> VSNAIKFIILTEIIFPTLLLVFGIYHGVMQVFYRSGIIKAESFLGIDYYQGLTLHGVINVIVYTTIFIVGFSNAIVAYSLKKPLREKVQWIALGMMVIGTLMAAWAMFTGRATVLYTFYPPLIAHWTFYLGAVLLVLGSLVPFFFDWIPSAIQWKRENPDQKLPLAVFGTFVNFILWTIMIVPVAIEILFQLLPLSLGLVDEINPLLARTLFWFFGHPVVYFWLLPAYVALYTILPKIVSEKGKLYSDPAARLAFILFLIFSLPVGLHHQFTDPGITNTWKLIHALFTFGVALPSMITAFTVATSLEYSVKAEHPELKNSKFYWWTFLPFMRLEGNKWMFSYFFAG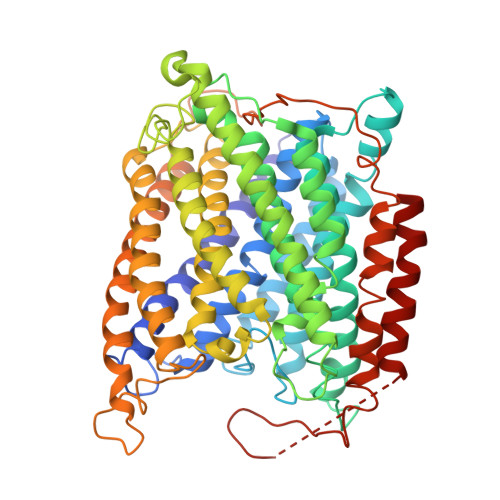LVLFFIGGITGIVNASYNVNLVVHNTAYVPGHFHTTVGGLVLLVFFALSLYMVSKLRGSEVKLKGLAVLAPYFWMQGMFMFSYAMMVGGVVVGFPRRTNAGLTYLNPDSPLYRPEWTGYAQLAAVGGVLLAIGFAFYFASLIATALAPKVRESTLEFPIADAYHDAPAPLLNNLKTWTVAAIILAVLSYIPPLYDASVRGVFFKSPAYNEKFPMPLKQLQGAEKKEEKKELSKAEGGITQK> SMMTSPIFDLSGRRALVTGASRGIGQSIAVALAEAGAHVAVTARTVEGLAETRALIEKTGRRAVALAQDVRDVEACASVTRAAAEGLGGLDILVNNAGF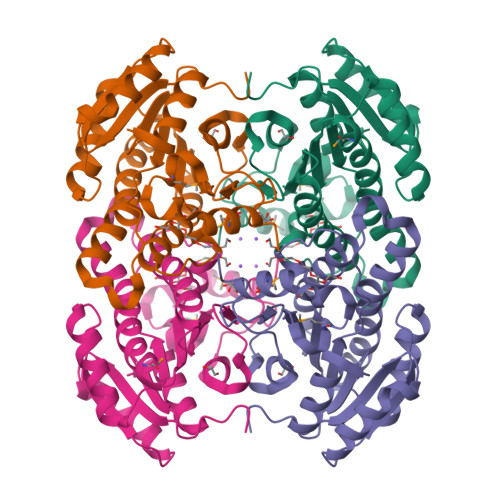ENVRPSFDVDEALWDTIVSTNLKGAFFCAQAAGRIMADANGGAIVNLCSLTSYVGIPTAVPYGASKSGLLGVTRALATEWAAHNIRVNAIAPGYFRTAMTAGFYEDEDWQSRMLEKIPQRRFGKESDIGGVAVFLCSDAAAYITGHCIPADGGYLASI>[4x]MAQSKGSVDQTLHAPHCEVGCAANVARRVGVDLARQVIGAHWASRMLVREVGTFPQPLLDRTQVTFSAQGEGWPALLARMTGGEVTSRHVPREELLSTLHADRAEGGTLLFMEDRACPWLDSAHSPGMLPHVVVPDGVAPDGSWQLIEGHSWWRGRYAMSEQDLLAASYPDPDPHHVAGRVLSLRIRPSAERAAQLD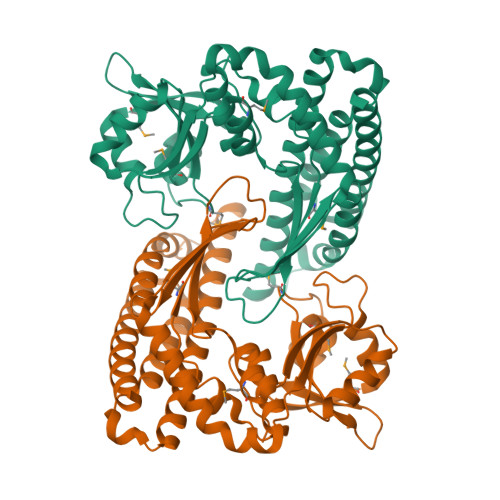TLARQELAAGLRTYLAAECGETETPAGRIVWANGPQSVPLLVERLRGWDYLCPLAARNDLSTEHARDVALGRYLFLALTDELAFAAYARAGTLRLVEGLGLAGAVGGLRPDEAWRLAWRSGQKLYRRLDRQNLSALFSALEKAAEVDVEYARRLLKELKLAAALEHHHHHHHH(2S)-2-amino-4-(2,3-dioxo-1,2,3,4-tetrahydroquinoxalin-6-yl)butanoic acid | C12 H13 N3 O4 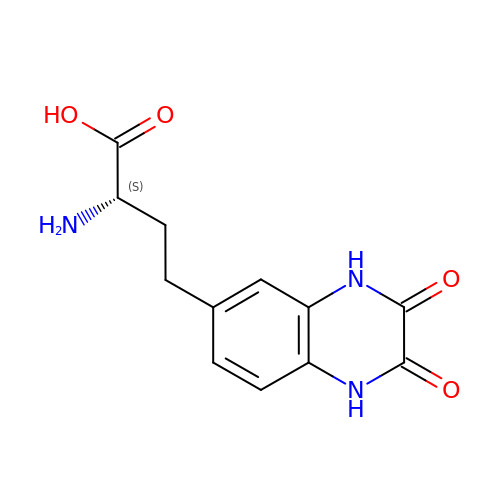| HOBORVHHDCBXLX-ZETCQYMHSA-N> MGKTNDWLDFDQLAEEKVRDALKPPSMYKVILVNDDYTPMEFVIDVLQKFFSYDV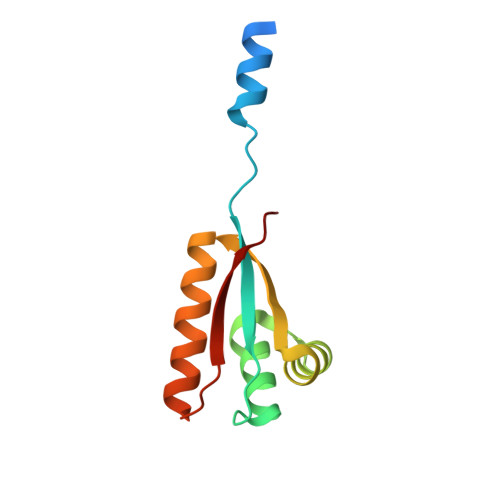ERATQLMLAVHYQGKAICGVFTAEVAETKVAMVNKYARENEHPLLCTLEKAGA> MSQSNRELVVDFLSYKLSQKGYSWS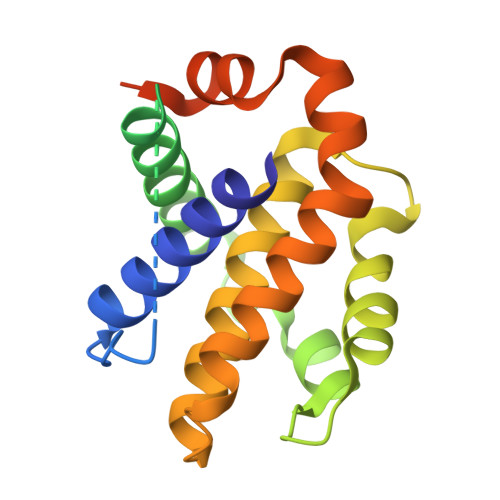QFSDVEENRTEAPEGTESEMETPSAINGNPSWHLADSPAVNGATGHSSSLDAREVIPMAAVKQALREAGDEFELRYRRAFSDLTSQLHITPGTAYQSFEQVVNELFRDGVNWGRIVAFFSLGGALCVESVDKEMQVLVSRIAAWMATYLNDHLEPWIQENGGWDTFVELYGNNAAAESRKGQERFNEHHHHHH> MLSKVKKVPSPYVGNLLNKWHDYIMQEKVHESIEKRTEIKQLLSQAEDNKDLVDYFILLDHRHSLCFDQEASMGDVVNMLSKGSHDLLINFYFELFAGDYEFFKKNYVKAISFYEKAEQKLSSIPNIEETKFAEFHYKIGVAYYEIDQHLVSVNKVTKARDIYKKSDMWNLEAIQCSLVVGINLYDMGRLDDADAYFRDALTEALDHGYDKPITKIYHNLGLVHWQKGSLELALHYFREAYSHEWLRDSPKGQQTVYMLSRVLYTMGQNEEAYHWYELGIEMARKFDDHEYKAKHDILYHLY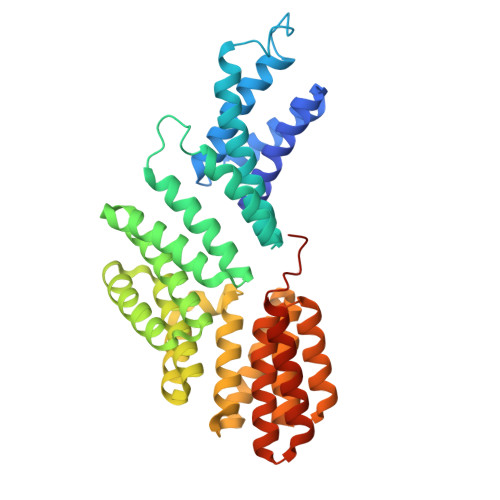EQPSIDEVKQSLAFLEERNLWPDVSKIAKGISELYEKKGDLVTSHEFLKRAFYAKEQIQRITEALGLEHHHHHH The essential enzyme messenger RNA (mRNA) (guanine-N7) methyltransferase catalyzes S-adenosylmethionine (SAM)-dependent conversion of GpppRNA ends to the m7GpppRNA cap structure characteristic of eukaryal mRNAs. The antibiotic sinefungin (SFG) is a SAM analog in which the S-CH3 sulfonium moiety of SAM is replaced by a C-NH2 amine. Available evidence indicates that the antifungal activity of SFG is exerted via inhibition of fungal cap methyltransferase Abd1. Crystal structures of K. lactis and S. cerevisiae Abd1 as binary complexes with SAH or SFG and ternary complexes with GTP•SFG highlight how SFG makes two hydrogen bonds from its C-NH2 amine to the guanine-O6 and -N7 atoms of GTP that account for its higher affinity vis-à-vis SAH and SAM.

We co-crystallized ScAbd1Δ140 with 0.7 mM SAH and determined the structure using KlAbd1Δ137•SAH as a search model. The final model was refined at 1.75 Å resolution with Rwork/Rfree of 16.4/18.6. The asymmetric unit contained one ScAbd1Δ140 protomer. Electron density for SAH was observed in the methyl acceptor site. ScAbd1Δ140 shares 83% sequence identity with KlAbd1Δ137. The two structures are superimposable with an r.m.s.d. of 1.1 Å over 289 Cα positions. All the atomic interactions of ScAbd1 with SAH recapitulate the interactions observed in the methyl donor site of the KlAbd1•SAH complex. The C-terminal 10-aa segment of ScAbd1 (aa 427–436), which is dispensable for activity and which is absent in KlAbd1, adopts a random coil conformation and projects away from the core methyltransferase domain.

> SSPIIKLRNFNNAIKYMLIDKYTKPGDVVLELGCGKGGDLRKYGAAGISQFIGIDISNASIQEAHKRYRSMRNLDYQVVLITGDCFGESLGVAVEPFPDCRFPCDIVSTQFCLHYAFETEEKARRALLNVAKSLKIGGHFFGTIPDSEFIRYKLNKFPKEVEKPSWGNSIYKVTFENNSYQKNDYEFTSPYGQMYTYWLEDAIDNVPEYVVPFETLRSLADEYGLELVSQMPFNKFFVQEIPKWIERFSPKMREGLQRSDGRYGVEGDEKEAASYFYTMFAFRKVKQYIEPESVKPN>AERPPEETLSLWKGEQARLKARVVDRDTEAWQRDPSFSGLQKVGGVDVSFVKGDSVRACASLVVLSYPELKVVYEDSRMVGLKAPYVSGFLAFREVPFLVELVQRLQEKEPDLMPQVVLVDGNGVLHQRGFGVACHLGVLTELPCIGVAKKLLQVDGLENNALHKEKIVLLQAG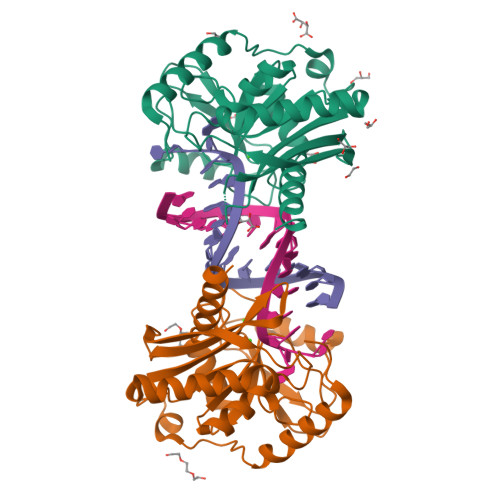GDTFPLIGSSGTVLGMALRSHDHSTKPLYVSVGHRISLEVAVRLTHHCCRFRIPEPIRQADIRSREYIRRTA[2x]>MAMKDLYVVNCCRTAIGSFGGSLKNTPAAEMGAVVVKEALKRANVAPENVDELMFGCILTSAQGQNVARQVSIKAGIPYSVPAYTVGMVCGSGMKSVIEGARSILAGDSDIVVCGGTENMSAAPFASMDARWGARMGDKKLVDTMIKDGLWDAYNNYHMGTTAENINDIWGITRREQDEFAAASQQKTEAAQAAGRFDDEIVPVMIKVKKEMVPFAKDEYPKAGVTADSIAKLKGAFPVGPESPNPVVVNTFEPTGCQDAPDKGTQRVTAANASGIN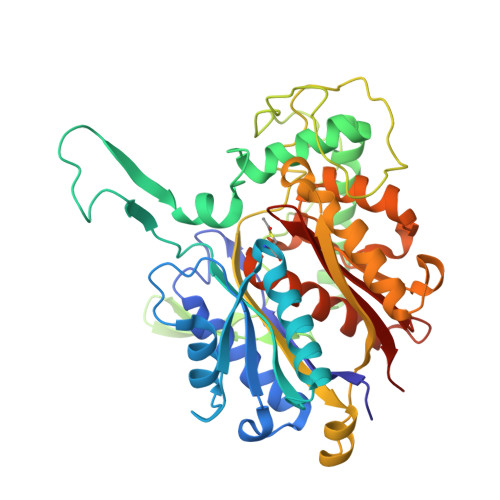DGAAAIVLASGEAVAKYGLKPMAKLIGWGQGGVDPKIMGVGPVVASRNAMKKAGVTIDDIDLIEANEAFAAQSIAVARELHFDMSKVNVNGGAIALGHPVGASGARIIVTLLHEMQKRPEAKKGLATLCIGGGMGTAVVFEKCLEHHHHHH[8x]> MVNSMFGGDLDPYEKSLNYEYPYHPSGNPKHIDVSEIDNLTLADYGWSPDAVKAYMFGIVVQNPDTGQPMGDEFYNHILERAVGKAERALDISILPDTQHEMRDYHETEFNSYMFVHAYRKPILQVENLQLQFNGRPIYKYPANWWKVEHLA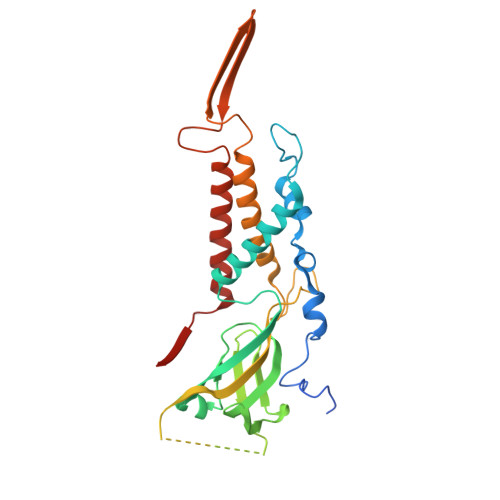GHVQLFPTALMQTGQSMSYDAVFNGYPQLAGVYPPSGATFAPQMIRLEYVSGMLPRKKAGRNKPWEMPPELEQLVIKYALKEIYQVWGNLIIGAGIANKTLEVDGITETIGTTQSAMYGGASAQILQINEDIKELLDGLRAYFGYNMIGL>[4x]MSKPIEIEIRRAPVLGSSMAYRETGAQDAPVVLFLHG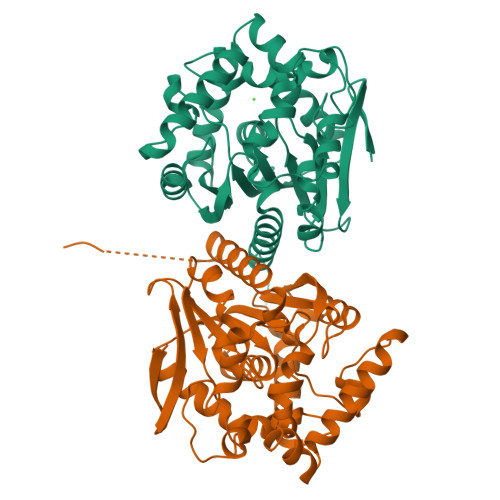NPTSSHIWRNILPLVSPVAHCIAPDLIGFGQSGKPDIAYRFFDHVRYLDAFIEQRGVTSAYLVAQDWGTALAFHLAARRPDFVRGLAFMEFIRPMPTWQDFHHTEVAEEQDHAEAARAVFRKFRTPGEGEAMILEANAFVERVLPGGIVRKLGDEEMAPYRTPFPTPESRRPVLAFPRELPIAGEPADVYEALQSAHAALAASSYPKLLFTGEPGALVSPEFAERFAASLTRCALIRLGAGLHYLQEDHADAIGRSVAGWIAGIEAVRPQLAAHHHHHH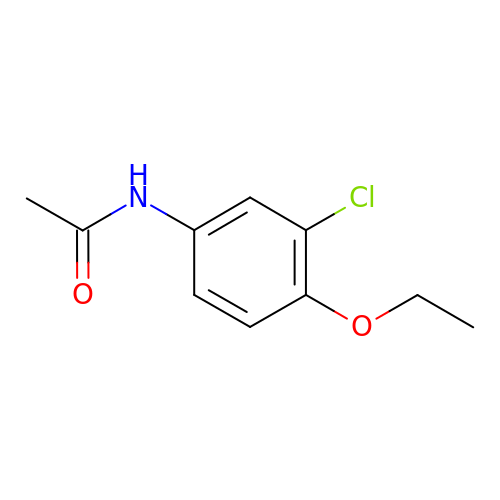~{N}-(3-chloranyl-4-ethoxy-phenyl)ethanamide | C10 H12 Cl N O2 | ORFOTXJLULZKSJ-UHFFFAOYSA-N> SFVKDFKPQALGDTNLFKPIKIGNNELLHRAVIPPLTRMRALHPGNIPNRDWAVEYYTQRAQRPGTMIITEGAFISPQAGGYDNAPGVWSEEQMVEWTKIFNAIHEKKSFVWVQLIVLGWAAFPDNLARDGLRYDSASDNVFMDAEQEAKAKKANNPQHSLTKDEIKQYIKEYVQAAKNSIAAGADGVEIHSANGYLLNQFLDPHSNTRTDEYGGSIENRARFTLEVVDALVEAIGHEKVGLRLSPYGVFNSMSGGAETGIVAQYAYVAGELEKRAKAGKRLAFVHLVEPRVTNPFLTEGEGEYEGG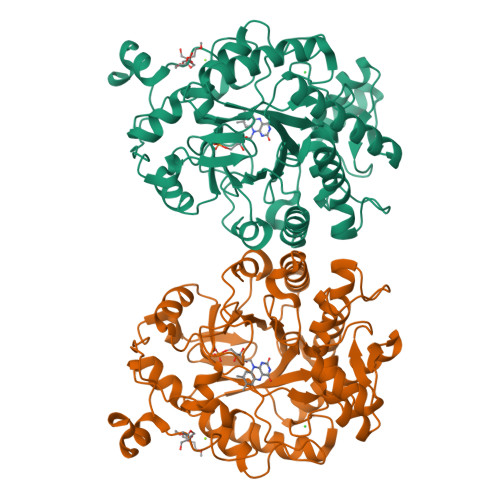SNDFVYSIWKGPVIRAGNFALHPEVVREEVKDKRTLIGYGRFFISNPDLVDRLEKGLPLNKYDRDTFYQMSAHGYIDYPTYEEALKLGWDKK> MSNNALQTIINARLPGEEGLWQIHLQDGKISAIDAQSGVMPITENSLDAEQGLVIPPFVEPHIHLDTTQTAGQ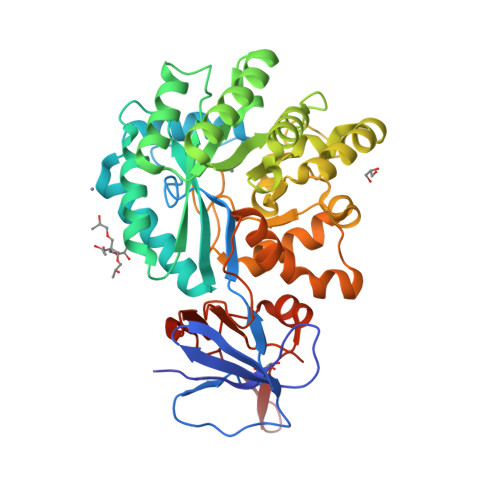PNWNQSGTLFEGIERWAERKALLTHDDVKQRAWQTLKWQIANGIQHVRTHVDVSDATLTALKAMLEVKQEVAPWIDLQIVAFPQEGILSYPNGEALLEEALRLGADVVGAIPHFEFTREYGVESLHKTFALAQKYDRLIDVHCDEIDDEQSRFVETVAALAHHEGMGARVTASHTTAMHSYNGAYTSRLFRLLKMSGINFVANPLVNIHLQGRFDTYPKRRGITRVKEMLESGINVCFGHDDVFDPWYPLGTANMLQVLHMGLHVCQLMGYGQINDGLNLITHHSARTLNLQDYGIAAGNSANLIILPAENGFDALRRQVPVRYSVRGGKVIASTQPAQTTVYLEQPEAIDYKR>[4x]GPLGSRRRVRAILPYTKVPDTDEISFLKGDMFIVHNELEDGWMWVTNLRTDEQGLIVEDLVEEVGR;>[4x]MHHHHHHSSGRENLYFQGSVFGVPLTVNVQRTGQPLPQSIQQAMRYLRNHCLDQVGLFRKSGVKSRIQALRQMNEGAIDCVNYEGQSAYDVADMLKQYFRDLPEPLMTNKLSETFLQIYQYVPKDQRLQAIKAAIMLLPDENREVLQTLLYFLSDVTAAVKENQMTPTNLAVCLAPSLFHLNTLKRENSSPRVMQRKQSLGKPDQKDLNENLAATQGLAHMIAECKKL

Deleted in liver cancer 1 (DLC1) is a tumor suppressor and ubiquitously expressed RhoGAP protein; its activity is regulated in part by binding p120RasGAP, a GAP protein for the Ras GTPases. RhoGAP proteins are key regulators of Rho family GTPases and influence a variety of cellular processes, including cell migration, adhesion, and cytokinesis. These GTPase activating proteins (GAPs) downregulate Rho signaling by binding and enhancing the intrinsic GTPase activity of Rho proteins. RhoGAPs enhance the intrinsically inefficient catalytic activity by directly binding the GTP-bound GTPase and contributing a conserved arginine residue, the so-called catalytic “arginine finger”, to stabilize the transition state of the GTPase enzyme active site and catalyze the reaction. One major binder and regulator of DLC1 is the RasGAP protein, p120RasGAP (RASA1; RasGAP, p120GAP). This was the first RasGAP identified and is a key regulator of Ras signaling. p120RasGAP is a multidomain protein containing two Src homology-2 (SH2), one Src-homology-3 domain (SH3), a Pleckstrin homology (PH) domain, presumptive calcium-binding C2 domain, and a RasGAP domain.

We determined the co-crystal structure to 3.2 Å resolution, and observe clear electron density throughout, including the key residues that mediate the protein-protein interaction. There are 4 copies of the DLC1-p120RasGAP complex found in the asymmetric unit, and they are experimentally identical (RMSD between 0.3 and 0.6 Å over 251 Cα atoms). We, therefore, determined the co-crystal structure of DLC1 RhoGAP domain in complex with p120RasGAP SH3 domain. This structure of a RhoGAP-SH3 interaction reveals that the RhoGAP domain cradles the SH3 domain in a manner competitive with its binding to RhoA. The p120RasGAP SH3 domain latches onto the DLC1 RhoGAP domain using its RT and n-Src loops and additional contacts are made between these latches by residues in the β2, β3 and β4 strands. On the RhoGAP domain, the bulk of the interface comprises residues on the solvent-accessible faces of αF and αG, with several more contributions from the αA-αA1 loop, αB, and the FG loop. Mapping the interaction regions on the surface of the two proteins reveals a single continuous binding site that buries a total surface area of 1550 Å2 comprising approximately 8% of the DLC1RhoGAP surface and 20% of the SH3 surface, with a shape complementarity score of 1.00 (Pisa server). The most notable feature of the RT loop binding is the direct interaction with the catalytic arginine finger residue Arg-1114 in DLC1 RhoGAP, located in the αA-αA1 loop. Specifically, Arg-1114 forms a salt bridge with the sidechain of Glu-298 and a hydrogen bond with the sidechain of Tyr-290, and additional van der Waals interactions with Val-293 in the RT loop and Trp-317 at the start of β3. We observe no material conformational change in either the SH3 domain or RhoGAP domain upon complex formation when compared to the previous apo structures.>[2x]REATWVTEKPLTLKIHMHFRDKWVWDENWPVAREVARLTNVKLVGVANRAA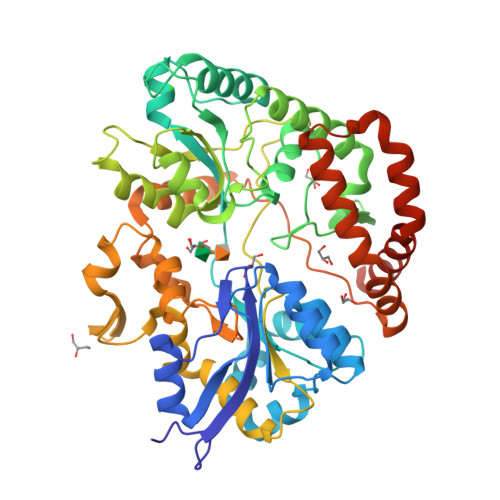TNSQEQFNLMMASGQLPDIVGGDNLKDKFIRYGMEGAFIPLNKLIDQNAPNLKAFFKTHPEVQRAITAPDGNIYYLPYVPDGLVSRGYFIRQDWLDKLHLKTPQTVDELYTVLKAFKEKDPNGNGKADEIPFINRDPEEVFRLVNFWGARSTGSNTWMDFYVENGKIKHPFAEVAFKDGIKHVAQWYKEGLIDPEIFTRKARSREQTFGNNIGGMTHDWFASTALFNDALSKNIPGFKLVPMAPPINSKGQRWEEDARQIPRPDGWAITATNKNPVETIKLFDFYFGPKGRELSNFGVPGLTYDIKNGKPVYKDTVLKAAQPVNNQMYDIGAQIPIGFWQDYEYERQWTNDVALQGIDMYIKNKYVLPQFTGVNLTVEEREIYDKYWPDVKTYMFEMGQSWVMGTKDPEKTWNDYQQQLKNRGFYQVMIVMQKAYDRQYGGAAKPAQVGAK> GGGGUUAUGUGUGCCCGGCAUGGGUGCAGUCUAUAGGGUGAGAGUCCCGAACUGUGAAGGCAGAAGUAACAGUUAGCCUAACGCAAGGGUGUCCGUGGCGACAUGGAAUCUGAAGGAAGCGGACGGCAAACCUUCGGUCUGAGGAACACGAACUUCAUAUGAGGCUAGGUAUCAAUGGAUGAGUUUGCAUAACAAAACAAAGUCCUUUCUGCCAAAGUUGGUACAGAGUAAAUGAAGCAGAUUGAUGAAGGGAAAGACUGCAUUCUUACCCGGGGAGGUCUGGAAACAGAAGUCAGUAGAAGUCAUAGUACCCUGUUCGCAGGGGAAGGACGGAA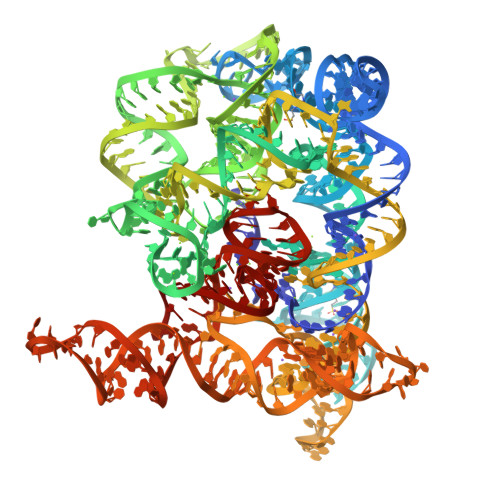CAAGUAUGGCGUUCGCGCCUAAGCUUGAACUGCCGUAUACCGAACGGUACGUACGGUAGUGUG> MEKDGLCRADQQYECVAEIGEGAYGKVFKARDLKNGGRFVALKRVRVQTGEEGMPLSTIREVAVLRHLETFEHPNVVR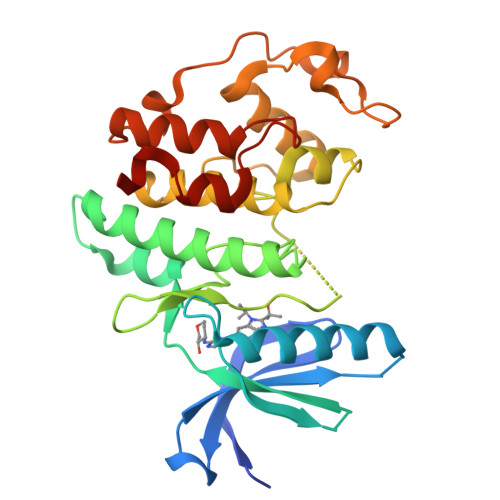LFDVCTVSRTDRETKLTLVFEHVDQDLTTYLDKVPEPGVPTETIKDMMFQLLRGLDFLHSHRVVHRDLKPQNILVTSSGQIKLADFGLARIYSFQMALTSVVVTLWYRAPEVLLQSSYATPVDLWSVGCIFAEMFRRKPLFRGSSDVDQLGKILDVIGLPGEEDWPRDVALPRQAFHSKSAQPIEKFVTDIDELGKDLLLKCLTFNPAKRISAYSALSHPYFQHHHHHH> AKLLEQIEKWAAETPDQTAFVWRDAKITYKQLKEDSDALAHWISSEYPDDRSPIMVYGHMQPEMIINFLGCVKAGHAYIPVDLSIPADRVQRIAENSGAKLLLSATAVTVTDLPVRIVSEDNLKDIFFTHKGNTPNPEHAVKGDENFYIIYTSGSTGNPKGVQITYNCLVSFTKWAVEDFNLQTGQVFLNQAPFSFDLSVMDIYPSLVTGGTLWAIDKDMIARPKDLFASLEQSDIQVWTSTPSFAEMCLMEASFSESMLPNMKTFLFCGEVLPNEVARKLIERFPKATIMNTYGPTEATVAVTGIHVTEEVLDQYKSLPVGYCKSDCRLLIMKEDGTIAPDGEKGEIVIVGPSVSVGYLGSPELTEKAFTMIDGERAYKTGDAGYVENGLLFYNGRLDFQIKLHGYRMELEEIEHHLRACSYVEGAVIVPIKKGEKYDYLLAVVVPGEHSFEKEFKLTSAIKKELNERLPNYMIPRKFMYQSSIPMTPNGKVDRKKLLSEVTALEHHHHHH

The D-alanyl carrier protein ligase DltA, as a remote homolog of acyl-(coenzyme A) (CoA) synthetase, cycles through two active conformations for the catalysis of adenylation and subsequent thiolation of D-alanine (D-Ala). In the first adenylation reaction, D-alanine is converted into DltA-bound D-alanine adenylate (D-Ala-AMP). In the subsequent thiolation reaction, the activated alanyl group in the intermediate is transferred to the thiol group of DltC-linked 4’-phosphopantetheine (DltC-SH). D-alanylation brings in positively charged amino-groups and partially neutralizes the net negative charges of the phosphate groups on the lipoteichoic acid backbone.

We also determined the structure of BcDltA in the absence of any substrate. The crystal structure of DltA in the absence of any substrate was observed to have a noticeably more disordered pocket for ATP which would explain why DltA has relatively low affinity for ATP in the absence of any D-alanyl carrier. The longest such disordered region is between Arg-397 and Glu-413, which contains the inter-domain hinge residue Asp-399, interacts with β-phosphate of ATP, and forms the pantetheine channel. Asp-399, equivalent to Asp-398 in BsDltA, serves as the hinge residue for domain rotation. The more disordered nature of the substrate-free conformation of BcDltA also implies that the previously observed adenylation and thiolation conformations are intrinsically unstable unless stabilized by the interaction with one or more substrates. This structural feature of BcDltA likely explains the relatively low sub-millimolar affinity for ATP, since part of the stabilizing BcDltA-ATP interactions would be used to compensate the cost of establishing the adenylation conformation of the protein.> MALEEIRPKEVYLDRKLLTLEDKELGSGNFGTVKKGYYQMKKVVKTVAVKILKNEANDPALKDELLAEANVMQQLDNPYIVRMIGICEAESWMLVMEMAELGPLNKYLQQNRHVKDKNIIELVHQVSMGMKYLEESNFVHRDLAARNVLLVTQHYAKISDFGLSKALRADENYYKAQTHGKWPVKWYAPECINYYKFSSKSDVWSFGVLMWEAFSYGQKPYRGMKGSEVTAMLE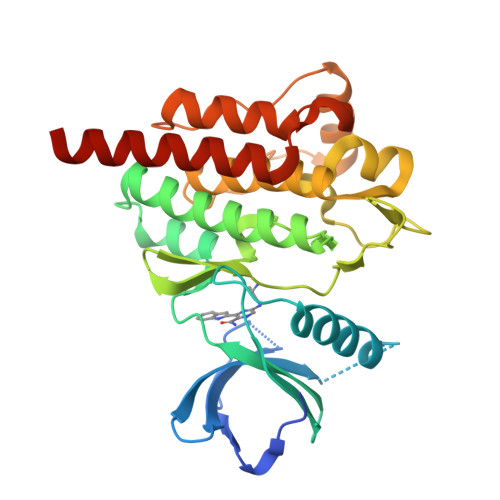KGERMGCPAGCPREMYDLMNLCWTYDVENRPGFAAVELRLRNYYYDVVNEGHHHHHH N-[4-[(6-chloro-[1,3]dioxolo[4,5-b]pyridin-7-yl)amino]-2-pyridyl]cyclopropanecarboxamide 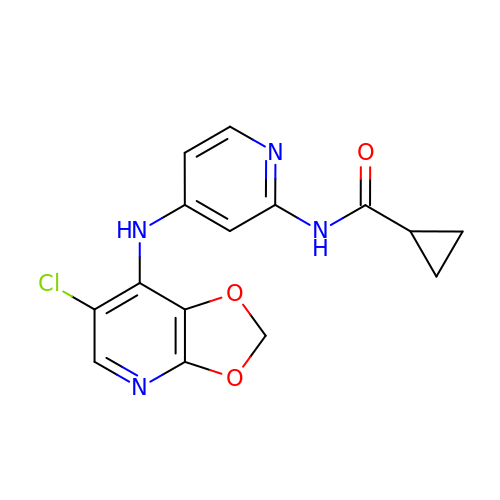| C15 H13 Cl N4 O3 | WJASKODGMHBDFO-UHFFFAOYSA-N5,6-DIHYDROURIDINE-5'-MONOPHOSPHATE | C9 H15 N2 O9 P | 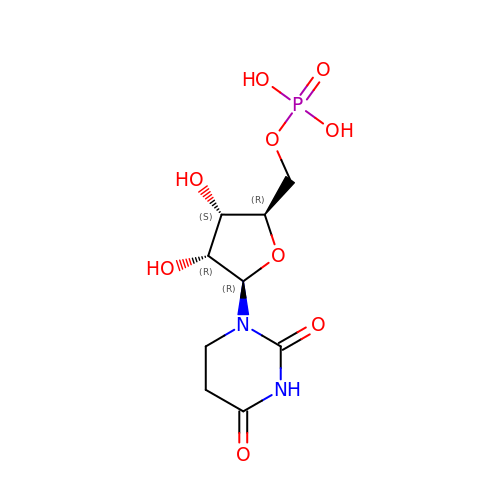NBWDKGJHOHJBRJ-XVFCMESISA-N> SPSVEACGYSDRIIQITRGDSTITSQDVANAVVGYGVWPHYLTPQDATAIDKPTQPDTSSNRFYTLDSKMWNSTSKGWWWKLPDALKDMGIFGENMFYHFLGRSGYTVHVQCNASKFHQGTLLVVMIPEHQLATVNKGNVNAGYKYTHPGEAGREVGTQVENEKQPSDDNWLNFDGTLLGNLLIFPHQFIN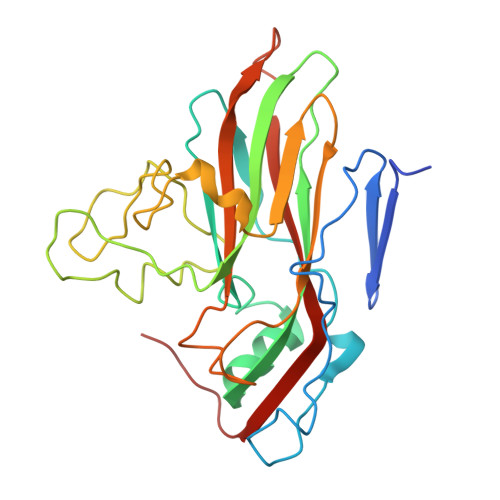LRSNNSATLIVPYVNAVPMDSMVRHNNWSLVIIPVCQLQSNNISNIVPITVSISPMCAEFSGARAKTVVQ> ACSVSASGTSSISVPSIYLMENGENSSQFNSGLSCTGFSLALANMTYLKYRVEQMSNSFTNAQTGEKLNAIILDSNNEIISLGQEKDMSSFTLVNLFSGPDGNLPFYIRLPAGQSVSPGVYQADSPLKVKWFYSVPAVAIVGIGVFFESPGFRRGALGIGFNWGSGADSLGSLSITVLPDCRILAQDVNFGTAAFASKLEPVQSSMGIRCSVNTPYYVSLNNGLSPQNGNQRAMKSQTGNTFLKYDIFKNSSNDRWGSGNERWS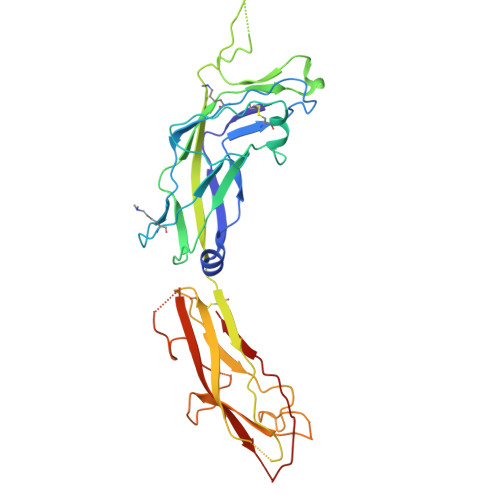SLNATINPGVHNGVTQQNYVFTTKIVDENADTIPAGTYQDTVTVQVEF> MSLSNHSSDIEVGHSMNLTNHFLVAMPSMKDPYFKRSVIYICEHNQDGAMGLMINAPIDITVGGMLKQVDIEPAYPQSHQENLKKPVFNGGPVSEDRGFILHRPRDHYESSMKMTDDIA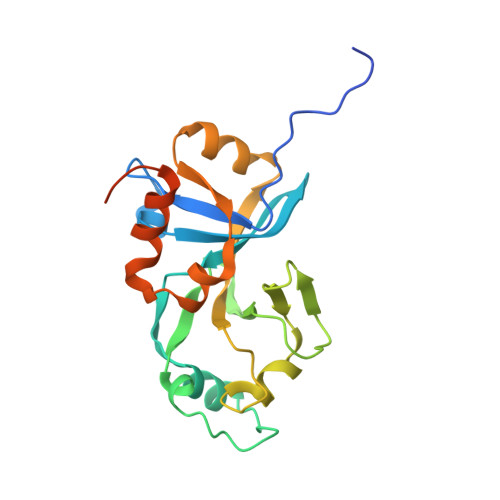VTTSKDILTVLGTEAEPEGYIVALGYSGWSAGQLEVELTENSWLTIEADPELIFNTPVHEKWQKAIQKLGISPAQLSSDAGHEGGSHHHHHH>[2x]MTDTDDGGTMLPLPDFTATFPEPFPAGPHSERTEHRLLDWLEEHPLLPSAKAKAVLVNITSHGASR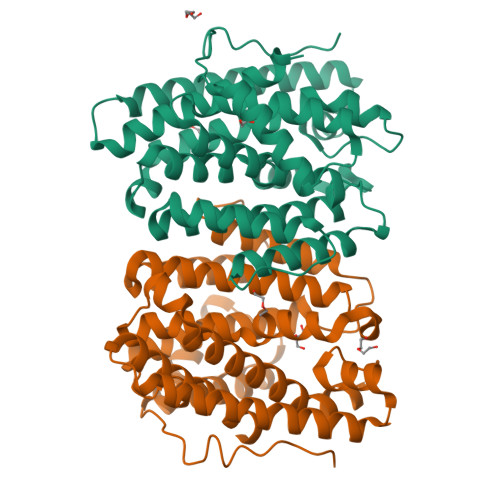TFPTADADDLLLFAELLLWLTAFDDVHAEGNGVGGPAALVDRASELMLVLAGGNPPRAMSPFPAVLHDLLARFRARASAAAYHRLAASLRDTLMALVWEAHHVAKPEGVALATYLAMRPHTVFIKTITAAGEILLGYELTDTQRALAAVRNLETAVANLAGWINDLASYEREMQRGRGQPLSLPTLLHARHGGTIEEAFTRASSMCENEAAVARRGITHLAHASPNALTAHARALEDITRSFIWHTSHARYQGIRPNRGSSTSSPARSLQHHHHHH The enzyme LkcE from the lankacidin polyketide biosynthetic pathway of the bacterium Streptomyces rochei represents an interesting test case for understanding such gain-of-function, as it exhibits a monoamine oxidase (MAO) protein fold yet also carries out a macrocyclization reaction. The catalytic mechanism proposed for LkcE involves initial oxidation of the amide function of LC-KA05 to an iminium ion. This is followed by attack of a C-2 enolate anion on the iminium to give the 17-membered lankacidinol A (2)8—an enzymatic intramolecular Mannich reaction.

The X-ray crystal structure of the holo protein was solved at 3.15 Å resolution by single-wavelength anomalous dispersion (SAD) using data collected on seleniated protein. The LkcE monomer contains two domains, a FAD-binding domain and a substrate-binding domain, which are joined by a substantial number of loop regions. The FAD cofactor is present at 100% occupancy, and as in other members of the MAO family, it adopts an elongated conformation. LkcE is clearly a homodimeric protein in the crystal, with an extensive interface (4705 Å2, representing 15% of the total surface area). In contrast, the dimer interface of LkcE is formed exclusively by the substrate-binding domain of each monomer. In all but the SeLkcE structure, one Gly (299 or 300) was an outlier, whereas Glu313 was an outlier in both forms of the holo enzyme structure.

>[2x]GPGSMTVVEAKSRIAVVGGGGSGSVAAWLLARRHDVTLFEADEYLGGHAYSHPVETDQGTLHVDMGVEHFNEKLSPNLFRLLTDFGIGTYVAPSSVHVDFPGEQQSWNNLDFLGELREELHEEFDRFHQEMNQLPTSGDDSYKQMSIGEYLDKHGYSKSFKYKAMNPILSIYSGCHAPSLDYNLMYVALSFSMNLLSFFSAGYWRKAQGGIHSYLARIESDLGERVRLNTPVEAVVPTQSGVTVLAGGQEHHFDQVVFATHADVTLRLLRTSDQQYRDLLGDFAYVPVESVLHQDESWLSPAGGGAYCQFRMPEGFELARAEEQMGSLTRNCNVLHPYRKVSSPILITFDPQEDVDPERVIVRREWKLPQLRPVDVRRKKRLHEIQGLNGLWFCGTDTSVTGHEGAIVSGMVIADRLGVPHPFPDDAPAAAQFRGIKEFMGV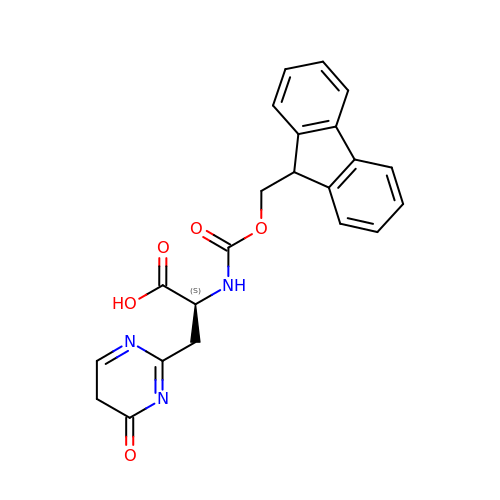(2~{S})-2-(9~{H}-fluoren-9-ylmethoxycarbonylamino)-3-(4-oxidanylidene-5~{H}-pyrimidin-2-yl)propanoic acid | C22 H19 N3 O5 | SRYLOGZQEQKDOT-SFHVURJKSA-N>MSSGKVIV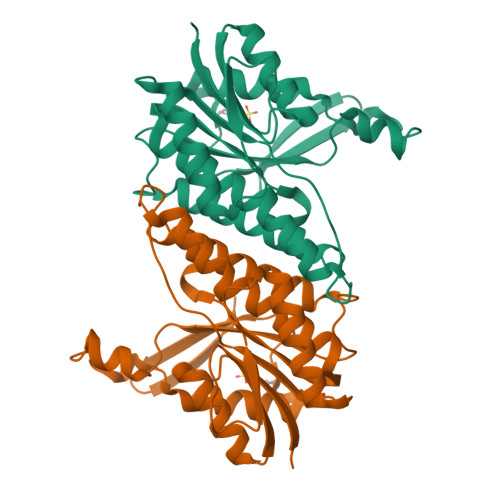YGGKGALGSAILEFFKKNGYTVLNIDLSANDQADSNILVDGNKNWTEQEQSILEQTASSLQGSQVDGVFCVAGGWAGGSASSKDFVKNADLMIKQSVWSSAIAAKLATTHLKPGGLLQLTGAAAAMGPTPSMIGYGMAKAAVHHLTSSLAAKDSGLPDNSAVLTIMPVTLDTPMNRKWMPNADHSSWTPLSFISEHLLKWTTETSSRPSSGALLKITTENGTSTITPQ[2x]>SLSSKDKDAVKALWGKIADKAEEIGADALGRMLAVYPQTKTYFSHWKDLSPGSAPVNKHGKTIMGGLVDAVASIDDLNAGLLALSELHAFTLRVDPANFKILSHCILVQLAVKFPKDFTPEVH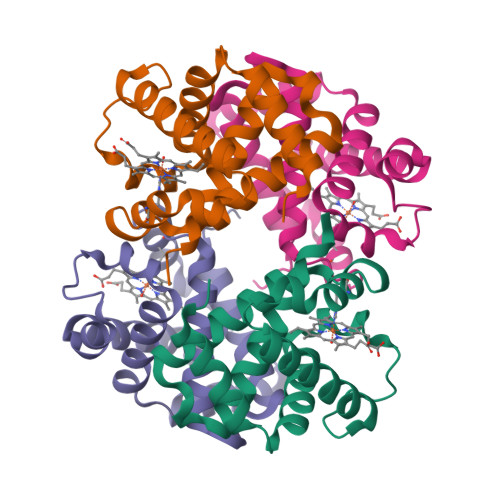LSYDKFFSAVARALAEKYR[2x];>[2x]VVWTDFERATIADIFSKLDYEAVGGATLARCLIVYPWTQRYFGNFGNLYNAAAIMGNPMIAKHGTTILHGLDRAVKNMDNIKATYAELSVLHSEKLHVDPDNFKLLSDCLTIVVAAQLGKAFSGEVQAAFQKFLSVVVSALGKQYH> ASMTGGQQMGRGSGPMLIEFNIPVDLKLVEQQNPKVKLGGRYTPMDGASVHKMALLVPFRDRFEELLQFVPHMTAFLKRQGVAHHIFVLNQVDRFRFNRASLINVGFQFASDVYDYIAMHDVDLLPLNDNLLYEYPSSLGPLHIAGPKLHPKYHYDNFVGGILLVRREHFKQMNGMSNQYWGWGLEDDEFFVRIRDAGLQVTRPQNIKT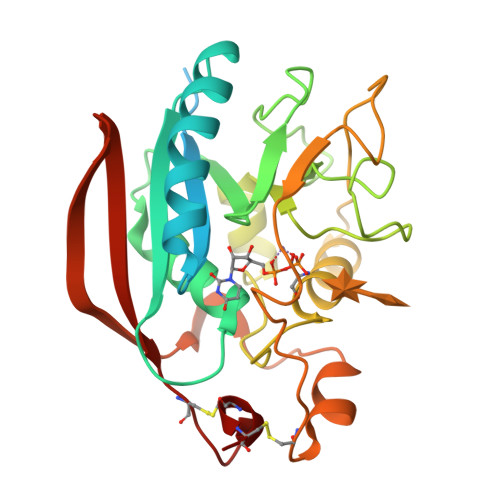GTNDTFSHIHNRYHRKRDTQKCFNQKEMTRKRDHKTGLDNVKYKILKVHEMLIDQVPVTILNILLDCDVNKTPWCDCS RamR is originally a transcriptional regulator from Salmonella typhimurium, which itself has no inherent catalytic function. Here, we report that a designer boron enzyme based on the transcriptional regulator protein RamR enables the kinetic resolution of hydroxyl thioesters by a boron-catalyzed hydroxide transfer reaction assisted by a nearby lysine residue. We incorporated a boron-containing amino acid into the protein scaffold RamR to create an active enzyme for the kinetic resolution of α-hydroxythioesters. We found that a closely positioned lysine residue is crucial for the catalytic activity of the designer enzyme by forming a hybrid catalytic dyad with the boronic acid residue.

Therefore, we analyzed the crystal structure of RamR_Y59pBoF (2.78 Å resolution, crystallized at pH 8.5). The overall structure is very similar to RamR without a boronic acid residue, but additional density at the para-position of the phenyl ring at position 59 clearly indicates the boronic acid residue, which seems to be mostly in the tetrahedral boronate form. A closer look into the hydrophobic pocket reveals multiple amino acid side chains in the vicinity of the boron residue, including a lysine residue at position 63. In the crystal structure, Lys63 lacks a clear electron density, indicating that its side chain is significantly disordered. However, the lowest energy side chain rotamer in a sterically favorable conformation available to Lys63 allows the formation of a direct interaction between the side chain ε-amino group and the boronic acid of pBoF (Nε(Lys63) to B(pBoF59) distance of ∼4.0 Å). Based on the crystal structure, the boron enzyme is in an equilibrium between boronate and boronic acid under catalytic conditions, most likely shifted to the respective anionic boronate species. In the 11B NMR spectrum, a chemical shift of 18.3 ppm for the boron residue was observed, mirroring the results of the crystal structure and indicating partial boronate formation under reaction conditions. Notably, the K63A mutation gave an inactive enzyme with a complete loss of catalytic activity (entry 3). Based on these observations, we believe that the canonical amino acid Lys63 and the noncanonical amino acid pBoF59 residue may form a hybrid catalytic dyad, in which the lysine acts similarly to serine/lysine dyads during the hydrolytic reaction catalyzed by certain serine peptidases. The term “hybrid catalytic dyad” refers to one canonical (Lys) and one noncanonical (pBoF) residue in designer enzymes that are in close proximity and are both essential for activity and selectivity in catalysis. Likely, Asp152 has an unproductive interaction with Lys63, and removal of this interaction leads to a large increase in catalyst activity.

>VARPKSEDKKQALLEAATQAIAQSGIAASTAVIARNAGVAEGTLFRYFATKDELINTLFLHLKQDLSQSMIMELDRSITDAKMMTRFIWNSYISWGLNHPARHRAIRQLAVSEKLTKETEQRADDMFPELRDLSHRSVLMVFMSDEYRAFGDGLFLALAETTMDFAARDPARAGEYIALGFEAMWRALTREEQAAWSHPQFEK[4x]>[2x]TKNPKLFISSTWMSHMTMPTENTDGEESLTSSKQQQQQSGDKHMEPLGTDDDFWGPSGPVSTEVVDRERNLYRVRLPMAGSYHCPSTGLHFVVTRAVTIEIGFCAWSQFLHETPLQHSHMVAGPLFDIKAEHGAVTAVCLPHFVSLQEGKVDSSLFHVAHFQDHGMVLETPARVEPHFAVLEN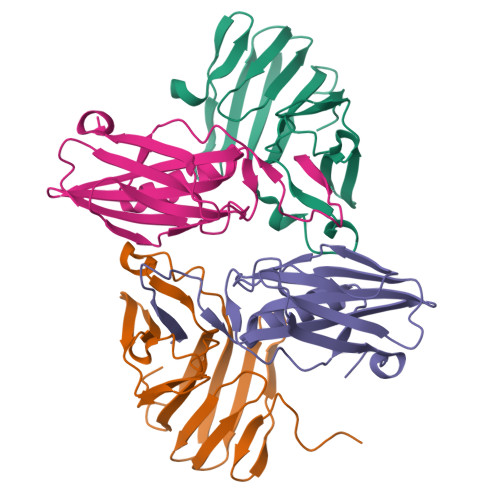PSF;>SPMGVLLRMIPAVGHFIPITSITLIYYRLYLEDITFHLYLVPNDCTIRKAIDEEELKFQFVRINKPPPVDALYVGSRYIVSSSKEVEILPKELELCYRSPRESQLFSEIYVGNIGSGINLQLTDKKYMNLIWEALLKPGDLRPALPRMASAPKD[2x]> MAG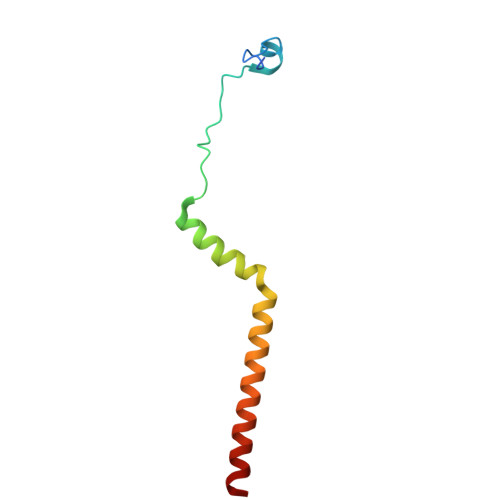GNYASLKADTSMDHVFGDSTNKLNYDFQLMSSKEAFFWNYTLYPIVGFPIFLYLYQFNKLENFEAEIAAAKAAKAASE> SQANLMRLKSDLFNRSPMYPGPTKDDPLTVTLGFTLQDIVKVDSSTNEVDLVYYEQQRW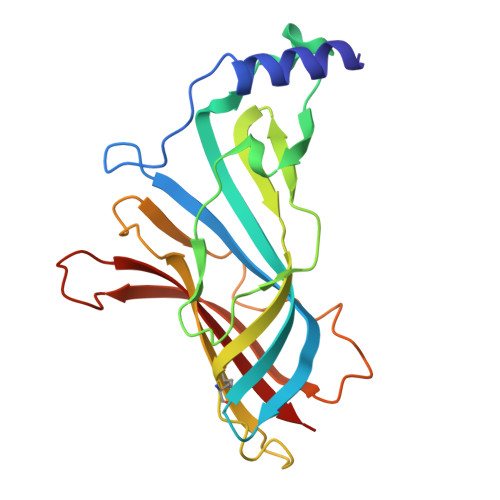KLNSLMWDPNEYGNITDFRTSAADIWTPDITAYSSTRPVQVLSPQIAVVTHDGSVMFIPAQRLSFMCDPTGVDSEEGVTCAVKFGSWVYSGFEIDLKTDTDQVDLSSYYASSKYEILSATQTRQVQHYSCCPEPYIDVNLVVKFRE> VAETPTYPW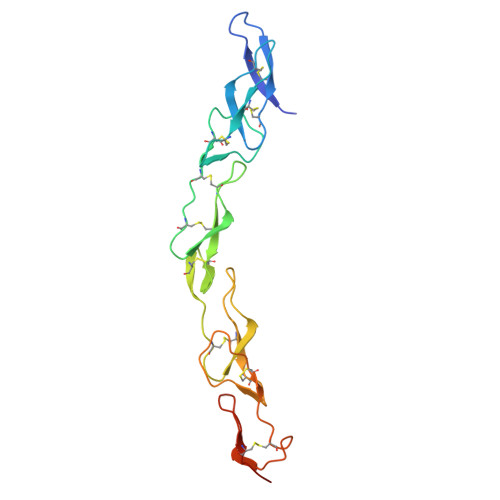RDAETGERLVCAQCPPGTFVQRPCRRDSPTTCGPCPPRHYTQFWNYLERCRYCNVLCGEREEEARACHATHNRACRCRTGFFAHAGFCLEHASCPPGAGVIAPGTPSQNTQCQPCPPGTFSASSSSSEQCQPHRNCTALGLALNVPGSSSHDTLCTSTGHHHHHH>MRKEEIKQAALTLFANNGFEGTSLADIAGVVGLKKQSIYSHFKDKDDLFLSIMKDAKSTEIDYYRAKLRDSDLSRPDLVLSSLLFGVKELYDTDEAYQFWLRYGFYPPKHLYEVVQADITENVLQMEHEFTDLFSNWMEQKLIPMQDVETMKEAYMGILDAVIVDIVYVNDPERTEKKITALWQIFWRGITLKALNL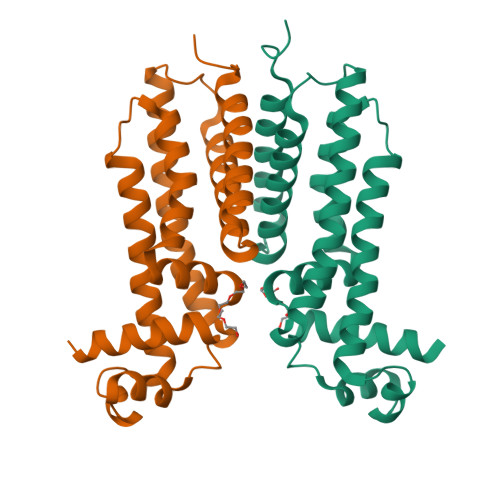EHHHHHH[2x]>[4x]SNAMADNINESEIIERLNSAPSVRGFFIATVDVFNESIDGLIQRIFRKDNFAVQSVVGPLLQDS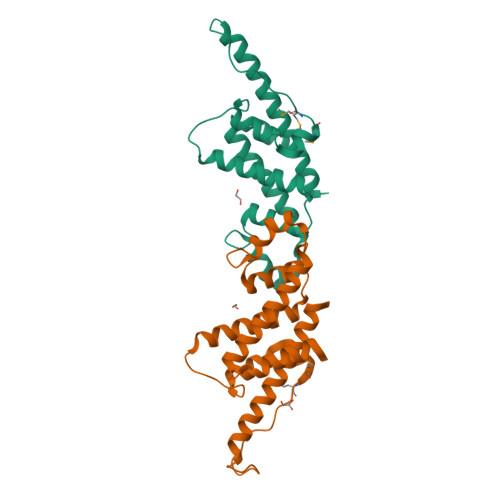GPLGDLSVRLKLLFGLGVLPDDIYHDIEDIIKLKNHLNSDASDYEFTDPNILEPIKKLHLVKKMGMVQLEVNEPDDDIDLEFYQLQLQRQQQIIKSGLSLAIVEICNELGK>MMFLRQEDFATVVRSTPLVSLDFIVENSRGEFLLGKRTNRPAQGYWFVPGGRVQKDETLEAAFERLTMAELGLRLPITAGQFYGVWQHFYDDNFS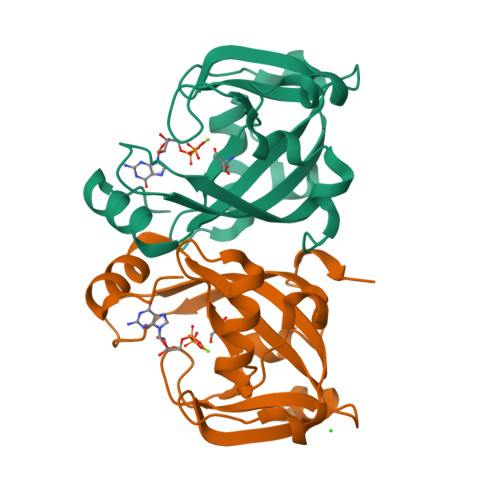GTDFTTHYVVLGFRFRVSEEELLLPDEQHDDYRWLTSDALLASDNVHANSRAYFLAEKRTGVPGL[2x]> MASMTGGQQMGRGSMSRDPLPFFPPLYLGGPEITTENCEREPIHIPGSIQPHGALLTADGHSGEVLQMSLNAATFLGQEPTVLRGQTLAALLPEQWPALQAALPPGCPDALQYRATLDWPAAGHLSLTVHRVGELLILEFEPTEAWDSTGPHALRNAMSALESAPNLRALAEVATQTVRELTGFDRVMLYKFAPDATGEVIAEARREGLHAFLGHRFPASHIPAQARALYTRHLLRLTADTRAAAVPLDPVL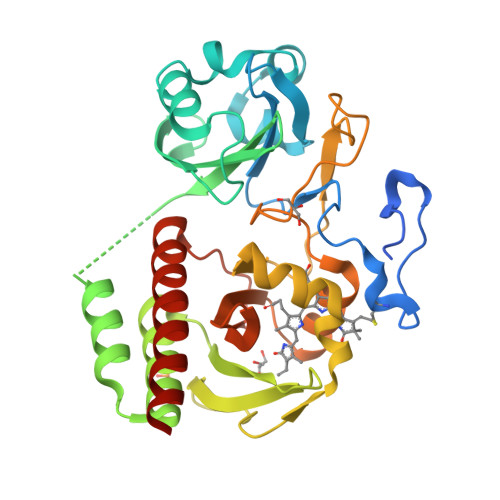NPQTNAPTPLGGAVLRATSPMHMQFLRNMGVGSSLSVSVVVGGQLWGLIACHHQTPYVLPPDLRTTLEYLGRELSEQVQVKEALEHHHHHH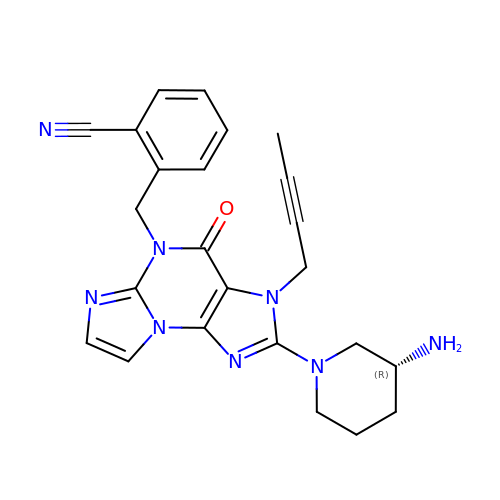2-({2-[(3R)-3-aminopiperidin-1-yl]-3-(but-2-yn-1-yl)-4-oxo-3,4-dihydro-5H-imidazo[2,1-b]purin-5-yl}methyl)benzonitrile | C24 H24 N8 O | FEXBDHCWKVFWPP-LJQANCHMSA-N>[3x]SNATGFLVSFMVDARGGSMRGSRHNGLRVVIPPRTCAAPTRITCRLVKPQKLS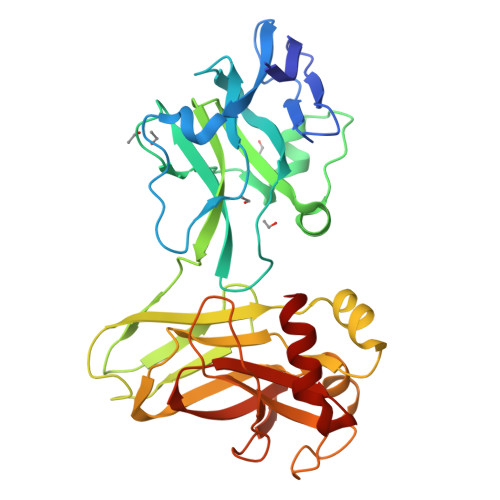TPPPLAEEEGLASRIIALGPTGAQFLSPVIVEIPHFASHGRGDRELVVLRSENGSVWKEHRSRYGESYLDQILNGMDEELGSLEELEKKRVCRIITTDFPLYFVIMSRLCQDYDIIGPEGGSLKSKLVPLVQATFPENAVTKRVKLALQAQPVPDELVTKLLGNQATFSPIVTVEPRRRKFHRPIGLRIPLPPSWTDNPRDSGEGDTTSLRLLCSVIGGTDQAQWEDITGTTKLVYANECANFTTNVSARFWLSDCPRTAEAVNFATLLYKEL> MAMSKSKVDNQFYSVEVGDSTFTVLKRYQNLKPIGSGAQGIVCAAYDAVLDRNVAIKKLSRPFQNQTHAKRAYRELVLMKCVNHKNIISLLNVFTPQKTLEEFQDVYLVMELMDANLCQVIQMELDHERMSYLLYQMLCGIKHLHSAGIIHRDLKPSNIVVKSDCTLKILDFGLARTAGTSFMMTPYVVTRYYRAPEVILGMGYKENVDIWSVGCIMGEMVRHKILFPGRDYIDQWNKVIEQLGTPCPEFMKKLQPTVRNYVENRPKYAGLTFPKLFPDSLFPADSEHNKLKASQARDLLSKMLVIDPAKR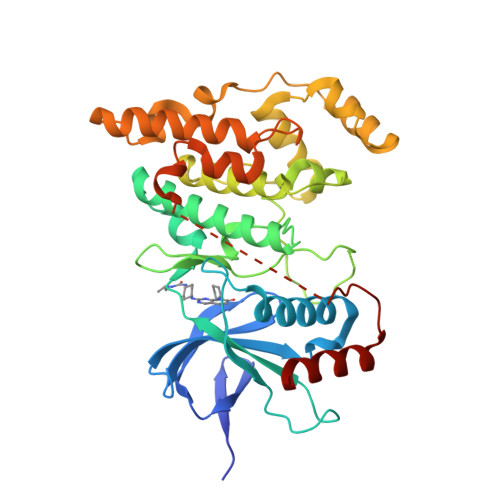ISVDDALQHPYINVWYDPAEVEAPPPQIYDKQLDEREHTIEEWKELIYKEVMNSE>CGTAAGGCG[2x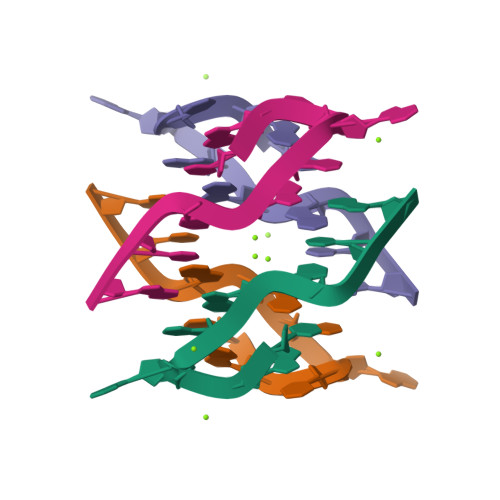]> MVMSKKIILITGASSGFGRLTAEALAGAGHRVYASMRDIVGRNASNVEAIAGFARDNDVDLRTLELDVQSQVSVDRAIDQIIGEDGRIDVLIHNAGHMVFGPAEAFTPEQFAELYDINVLSTQRVNRAALPHMRRQKHGLLIWISSSSSAGGTPPYLAPYFAAKAAMDAIAVQYARELSRWGIETSIIVPGAFTSGTNHFAHSGVPDDHARQAEYEAGPNAGLGEEIKKAFAAIVPPDADVSLVADAIVRVVGTASGKRPFRVHVDPAEDGADVGFSVLDRLRAEMLHRVGLSDLLKPRALAAENLYFQS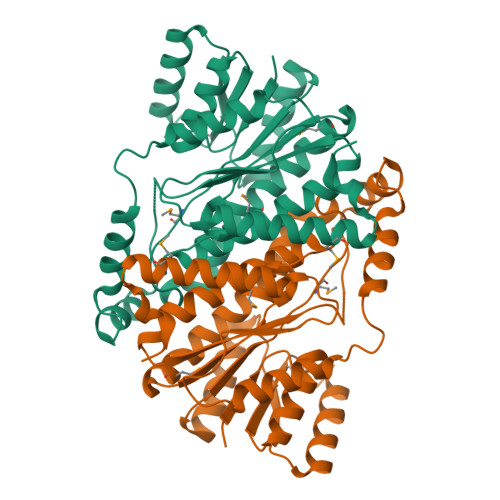HHHHHHWSHPQFEK>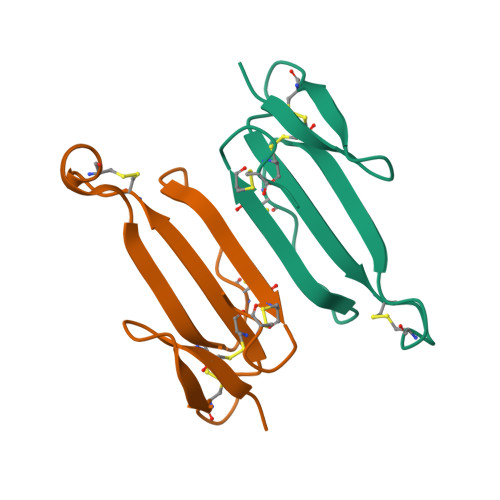MRTCLISPSSTPQTCPNGQDICFLKAQCDKFCSIRGPVIEQGCVATCPQFRSNYRSLLCCTTDNCNH[2x]>MAPITAYSQQTRGLLGCIITSLTGRDRNQVEGEVQVVSTATQSFLATCVNGVCWTVYHGAGSKTLAGPKGPITQMYTNVDQDLVGWQAPPGARSLTPCTCGSSDLYLVTRHADVIPVRRRGDSRGSLLSPRPVSYLKGSSGGPLLCPSGHAVGIFRAAVCTRGVAKAVDFVPVESMETTMRASKKKKKGSVVIVGRIILSGRK[9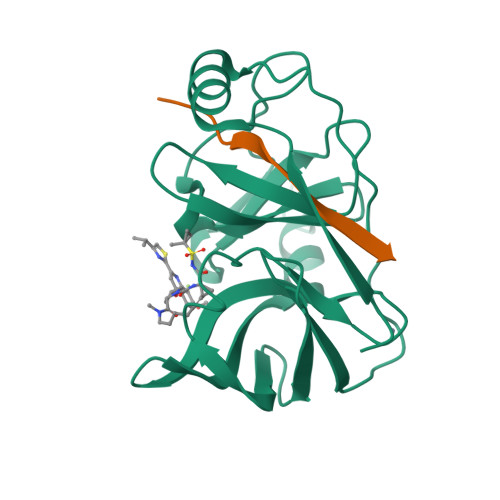x];>KGSVVIVGRIILSGRK[9x]>[3x]MSLGKFLVEREQMRYPVDVYTGKIQAYPEGKPSAIAKIQVDGELMLTELGLEGDEQAEKKVHGGPDRALCHYPREHYLYWAREFPEQAELFVAPAFGENLSTDGLTES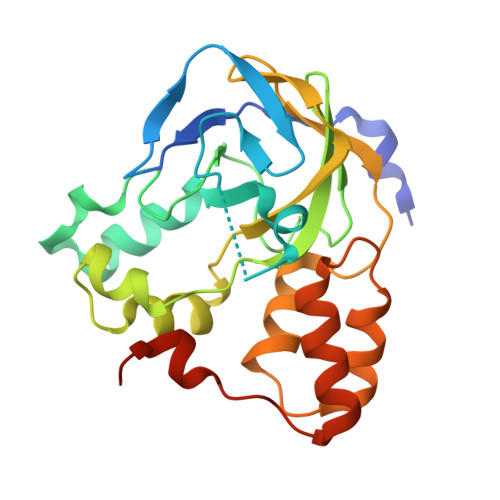NVYMGDIFRWGEALIQVSQPRSPCYKLNYHFDISDIAQLMQNTGKVGWLYSVIAPGKVSADAPLELVSRVSDVTVQEAAAIAWHMPFDDDQYHRLLSAAGLSKSWTRTMQKRRLSGKIEDFSRRLWGKEGGSHHHHHH>[2x]MGKASVDQISKLMKVSSSVVENHPPSPQISDQGAKVPLVKGVGERNLSIYRHSDGRVEVVVSPPPPAHLVLSGGGAKGIAFPGMVQALEEADKLKGVKVVSGSSAGAICAALLASGMDAKAFTQLSNNLDLPRLLNSKDPVTAWLQEASSELGKLVRSLPGPVGNISQLLLTLLPRLQTEGQPLEDLIRNESRQSILAHIAGMPPANRPPEVTAIAERLSAGGGATFRDLEV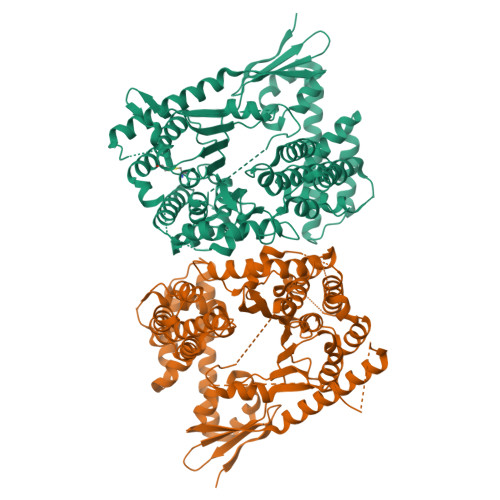LSRHIPAIKQLNITGTGMFDGRPQLVVFNANLTPDMDIGRAALISGALPGLFKSPTEQGHGFQAASQVTAFQDGGLLLNTPAPGVIERSFPESPLGKDEALIVKFESDKASAPPRSGGFFSFLADTFTGTPHTAAESYQNDRLQAFSEQTVTLPLNSDKGDFRGLLDGTVNFTMTPEQKQHLQAQARQTVSGHLQQRELERERHEFPSLNDAVMAMDDQMLASVQVDLQNDAAGAEALRFRKDAQQALQALDTAIAEANQTSTSLVITPKLASALRNLDALARRPEDIEWLGKRLNAPGQRNFQQLLQVGTKQASSNGSGLSKVLTSAVAEMQKRDIGVKAENFIREVIYPSLYRPGQPAANVELLQRAVRDLGEATTPAEFNRVLDGIVKHYRARNKPWSKPFSSTTVEQAKAWRIPVGGRLVPRGSPGAAGHNHNHNHNHNHN>[6x]MENQLFIIGIGTGTDEYENFEETILKGVKRNELEGQIGPDILDNCCSDVCYFWGRSKETIYEKKIDKGDMVLFYVGKRISRNKVDLNQETAVYLGIICETVEISENDVSFLNDFWRKGENFRFLMFFKKKPEKLHHSINEINSKLGYNPDYFPIAGYVKPERMSGVYDILKNILKKRGILKESDSMNESAGHNIKEDYFRVDMLLNKKGQVILYGPPGTGKTWIARKYVVEETNEKTPGNKWEFITFHQSYSYEEFIEGFRPRTDNEEKIRYVVEDGIFKKIALRALVKGLFELEDATIGKDKIHRLYILLTKKEPLSPTEYEEYLRLKRYLWELVGGLPKDKLKNLTPKFYLIIDEINRGNISKIFGELITLLEKDKRLGGENQLIVRLPYSGEPFAVPPNLYIIGTMNTADRSIALLDVALRRRFAFIEVEPRPEFLEKENLKKIREKKLKTEDRKRLNEKLNELFSKLGNDNYFLKTLLEKINVRITVVKDRDHRIGHSYFLNVETVEDLHHVWYYEVLPLLMEYFYNDWETIKWVLNEKGKEHGNVFFEKLRLTGPNGEEAYQLKVLEGDAFIGALKRIISKNTPSQEGGATTNEENSPENTQSQTEGD;> MPRLTTITLYEHDEKRYRDIAGDKKAIQDALIKLNKQFKKDFKKLDRSEDNSDTEDTIDESKGVVEVYANKIKARHYVGFAAVDNVFLQILPKVFKPKKEQTQETQEDTWEPILAFIRMLDMAYGLKIKDHDLAYLQGRNLRPNLYEVFIYLFAKSLWSEVQRGYHREYVEVHREEKFLRGKLLMSRQIRKLPHQLNTFSVEVHELIEDNLLNRIFYASVREAL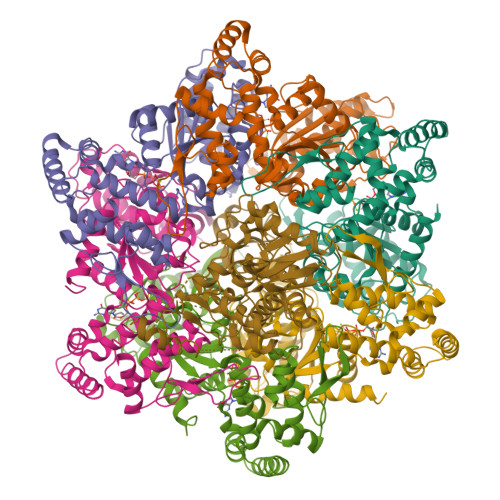RRTTWGLNRKLLGELMLAFDGITPIHLRTEHFERVHFTRLNERFRRPFELAKLLFMPASGKGRSREVSGFFVDMNKLFERFIERVLVRNLPPEYKLFYQESYPFLKNQNGSSQKPDYVVRKGNTPVVVLDAKYRELKERIPSSDMLRQLYVYSRIWGYKTSHENDSKPPAVIVIPSSSTYNQGLPDKPLEFEFFDERKLFIVAYNMDYVKTGAIFKADKNFRRSLNNIIGKLNT>MATDRQLAEEYLYRYGYTRVAEMRGESKSLGPALLLLQKQLSLPETGELDSATLKAMRTPRCGVPDLGRFQTFEGDLKWHHHNITYWIQNYSEDLPRAVIDDAFARAFALWSAVTPLTFTRVYSRDADIVIQFGVAEHGDGYPFDGKDGLLAHAFPPGPGIQGDAH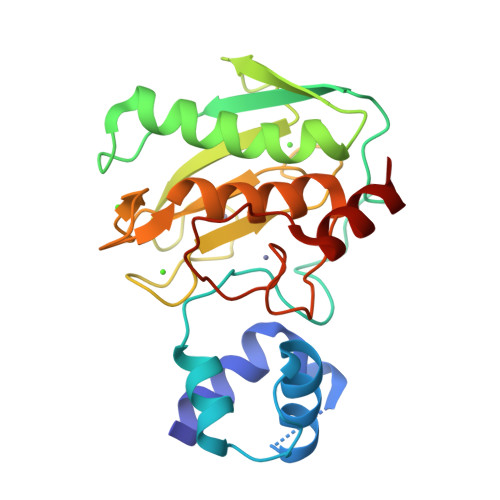FDDDELWSLGKGQGYSLFLVAAHEFGHALGLDHSSVPEALMYPMYRFTEGPPLHKDDVNGIRHLY[4x]> SPDKKWLGTPIEEMRRMPRCGIRLPLLRPSANHTVTIRVDLLRAGEVPKPFPTHYKDLWDNKHVKMPCSEQNLYPVEDENGERTAGSRWELIQTALLNKFTRPQNLKDAILKYNVAYSKKWDFTALIDFWDKVLEEAEAQHLYQSILPDMVKIALCLPNICTQPIPLLKQKMNHSITMSQEQIASLLANAFFCTFPRRNAKMKSEYSSYPDINFNRLFEGRSSRKPEKLKTLFCYFRRVTEKKPTGLVTFTRQSLEDFPEWERCEKPLTRLHVTYEGTIEENGQGMLQVDFANRFVGGGVTSAGLVQEEIRFLINPELIISRLFTEVLDHNECLIITGTEQYSEYTGYAETYRWSRSHEDGSERDDWQRRCTEIVAIDALHFRRYLDQFVPEKMRRELNKAYCGFLRPGVSSENLSAVATGNWGCGAFGGDARLKALIQILAAAAAERDVVYFTFGDSELMRDIYSMHIFLTERKLTVGDVYKLLLRYYNEECRNCSTPGPDIKLYPFIYHAVESCAETADHSGQRTGT

PARG, a single gene alternatively spliced to generate five isoforms, is an endo- and exo-glycohydrolase that rapidly degrades PAR generated by PARP1 to coordinate DNA repair. PARG hydrolyzes α(1′′-2′) O-glycosidic linkages in PAR chains to release ADP-ribose and oligo(ADP-ribose) chains that may signal genotoxic stress. The hPARG active site has two deep pockets that specifically engage the adenine and diphosphate group of ADPR. Our high-resolution crystal structures of human PARG bound to these methylxanthine inhibitors revealed detailed interactions that support a mechanism of competitive inhibition.

JA2131/NSC98003 contains a terminal morpholine in place of the pyrrole of JA2-4 and shows improved activity, which may derive from a polar interaction mediated by the 1´-oxygen of the morpholine. The 6´-thiocarbonyl group of JA2131 is another driver of inhibitory potency. JA2131 and JA2120 bind to the adenine-binding pocket of hPARG in the same orientation as JA2-4. As for JA2-4, the 6´-thiocarbonyl of JA2131 makes a direct van der Waals contact with the main chain amide of Asn869 (3.6 Å) from the conserved macrodomain fold. The morpholine oxygen of JA2131 appears to accept a hydrogen from the side chain amine of Asn869, explaining the modest increase in potency compared to JA2-4. Notably, the 6´-thiocarbonyl group of JA2-4 series inhibitors displaces this water molecule to form improved interactions with the adenine-binding pocket of hPARG. From the protein-ligand interactions identified here, the 6´-thio-methylxanthine derivatives JA2-4 and JA2131 compete with the adenine moiety of PAR substrates for active site binding. The results show JA2131 treatment induced a 9 °C stabilization of PARG proteins in cells; whereas, the PCNA control showed no significant change in thermal stability in response to JA2131 treatment. JA2131 did not inhibit PARP1 activation up to 100 μM; whereas, a potent PARP inhibitor Olaparib completely shuts down PAR synthesis by PARP1. These results, together with the observed extensive physical interactions between JA2131 and its binding site on hPARG, support the conclusion that JA2131 selectively inhibits PARG activity.> MEGFLNRKHEWEAHNKKASSRSWHNVYCVINNQEMGFYKDAKSAASGIPYHSEVPVSLKEAICEVALDYKKKKHVFKLRLSDGNEYLFQAKDD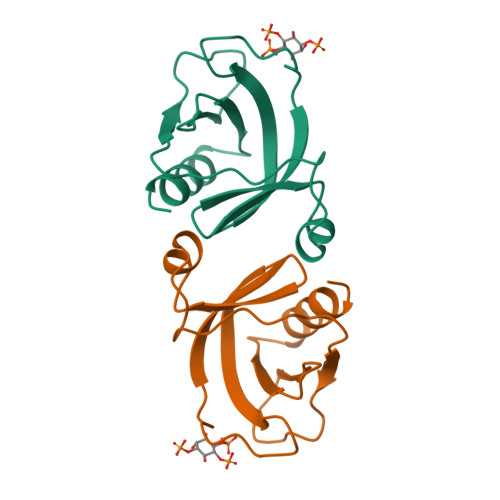EEMNTWIQAISSA> ERKVEKLLVANRGEIACRVFRTCREMHIRTVALFCEAERNAKHVAEADEAVCIGPPPAVNSYLRGEHIISVAKQLNVDAIHPGYGFLSENASFADAITRSGIEFIGPPASAISLMGSKSESKRIMEAAGVPVVPGYYGENQNVSFLAEEAKKVGFPILIKAVSGGGGKGMKIVERPEDFTFMLESAKREATNFFKDDRVILERYVKRSRHIECQIFFDKHGRGVFFFERDCSVQRRYQKVLEEAPAPHLSMETRQRIGEVALQAAKAVGYVGAGTVEFIFDTSTGEFYFMEMNTRLQVEHPVTEEVCRIKGAPLDLVKLQIKTAMGKPLTFSQEDVTLVGSCIEARVYAESPERGFLPESGPLTFIREPFQGVRGPARTRLDTGFREGDNVLIHYDPMLAKVISWGRSREEALRGLRQALGEYKVAGINTNIEFLKRCCETPEFARGGVTTNFISEHESQLLKSPVVTPEVAAMAATAWLLNRCDNWRGAFRLNSDTNATVHFYIDDHPVEVRLHTEGANYHKIFFSVWDHDGSFEVCSGPVTSKHRDQKSIVNDFTFLFENGMHHTVLAVATEGDVTVIGSFGLHQ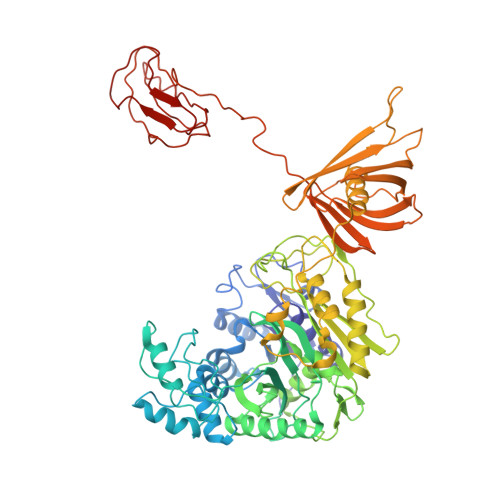LRLLPLTDGFGDSSTAGGTSTKIVSPMPGKVSKLLVKSGDLVEKGQVLVIVEAMKMEHPVRALQDGRVSFLVKEGEVVGGDHVLATVAEEE> MTRQAYSSMLLSTAAALTLAFSLNASAAVDVDAAKSLARENNCFKCHGVDKEKDGPSYKKVAEKYRGKADAEAKLIHHVTSGEKAKFPDGHEEEHKNINGKASPEAIKNLVDWILSLWSHPQFEK

In summary, the structure and electrochemical properties of MtoD are consistent with its possible role as an electron shuttle between MtoAB on the outer membrane and a range of potential electron acceptors on the inner membrane. Further analysis of the sedimentation data gave a f/fo coefficient of 1.24, indicating that MtoD behaved like a monomeric globular protein in solution.

The crystal structure of MtoD was solved to an initial resolution of 2.29 Å by single wavelength anomalous dispersion (SAD) using the anomalous signal caused by the single iron atom contained within the heme group. The initial model was used as a template for molecular replacement to obtain a final resolution of 1.47 Å. The crystal structure contained residues 28–119 of the processed amino acid sequence and a single c-type heme covalently attached to Cys43 and Cys46 via thioether bonds, consistent with the histidine ligands predicted from the sequence alignment. The imidazole side chains of the two histidines coordinating the heme iron are arranged near-parallel relative to one another, at an angle of approximately 35°. One obvious difference is that the axial coordination of the MtoD heme is bis-Histidine, while other crystallized cytochromes have Histidine/Methionine coordination. The class 1 cytochromes typically contain a flexible loop that covers the front of the heme, however in MtoD this region is restrained by a hydrogen bonding network that causes the formation of a β-loop and prevents the peptide sidechains from interacting with the heme propionate groups. This causes an increase in the overall surface exposure of the MtoD heme, giving an overall exposed heme of 152 Å2 compared to 30–61 Å2 for other class 1 cytochromes. To date the heme group of MtoD is significantly more exposed to solvent than the heme of any other structurally resolved monoheme cytochrome, suggesting that the properties of the heme are likely to be extremely susceptible to changes within the local environment. The measured redox potential of +155 mV for the MtoD heme is high for a bis-His coordinated heme and the heme group is significantly more solvent exposed than in monoheme cytochromes. Previous studies on the potentials of the heme groups of MtoA indicate that they span a mid-point potential range between +30 and −350 mV, which is lower than the potential of MtoD and indicates that electron transfer from MtoA to MtoD would be thermodynamically favorable. This supports the hypothesis that MtoD could be the electron transfer shuttle between the outer membrane MtoAB complex and the cytochrome bb3 oxidase on the cytoplasmic membrane, allowing the efficient generation of a PMF.> GSGSRPHLAGTHTSLRLPQEGKGTCILVGGHEITSGLEVISSLRAIHGLQVEVCPLNGCDYIVSNRMVVERRSQSEMLNSVNKNKFIEQIQHLQSMFERICVIVEKDREKTGDTSRMFRRTKSYDSLLTTLIGAGIRILFSSCQEETADLLKELSL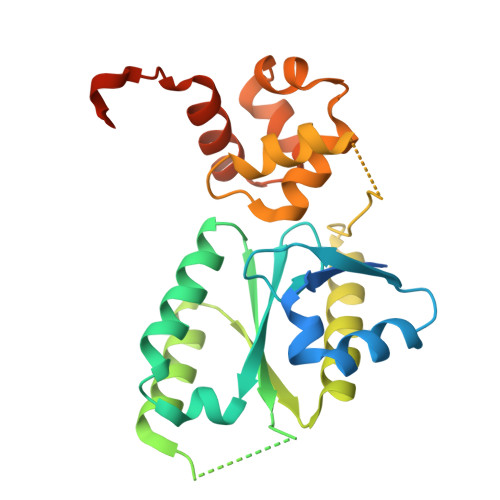VEQRKNVGIHVPTVVNSNKSEALQFYLSIPNISYITALNMCHQFSSVKRMANSSLQEISMYAQVTHQKAEEIYRYIHYVFDIQMLPNDLNQDRLKSDI>[2x]GHMAV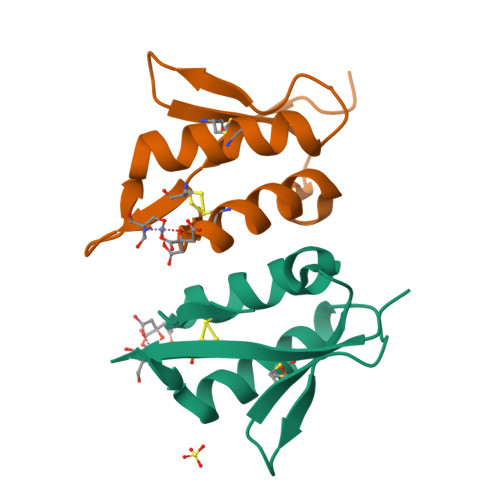VYAARCKFGNPLVQNNRITRAVCDLTNEHTTKDGSWHYVEVDNECKYLAGDNPRDQPGWAVFVKYCTYYKGVPDA>[2x]FPDNAVPYPWSNAQLSWQRTAFHFQPERSWMSDPDGPIFYKGWYHFFYQYNPDNPVWGNNTWGHTVSRDLIHWLYLPLALAADQWYDMQGVFSGSATCLPDGRIMMLYTGVTKEMVEMLSLAYPADLSDPLLVEWVKYPGNPILSAPPGVSPTEFRDASTGWYVSNGTWRIAIGAKYNTTGIAMVYETKDFKSFKLLEELLHAVPDTGLWECVDLYPVSTTGEKGLETSVNGPKVKHV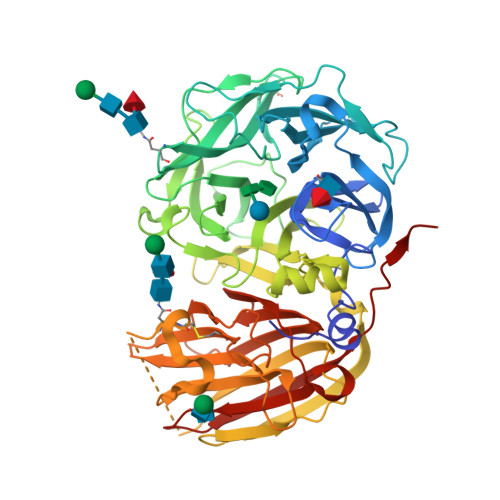LKASIDEQQRDYYAIGTYDLGTNKWTPDNPEEDVGIGLRYDWGKYYASKTFYDPKKQRRVVWAWTKELDSEVADREKGWANVQTIPRTVLLDQKTGTNVLLWPVEEVESLRLSSKEFSKVKAGAGSVVPLDVGTATQLDIIAEFEIDKEALEGTIEADMGYNCTTSGGAAERGVLGPFGLLVSATENLSEQTPVYFYIAKGTDGNFKTFFCLDESRSSKASDVSKQVKGFTVPVLDGEKFTMRLLVDHSIVESFAQGGRSCITSRVYPTEAIYGAAKLFLFNNATGASITASLKIWEMNSAFIQPFHR1-naphthalen-2-ylethanone | C12 H10 O | 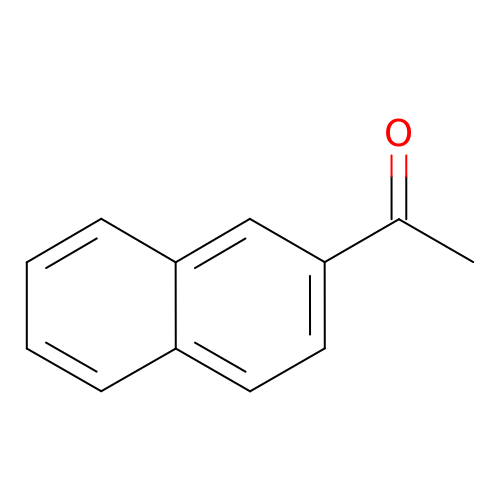XSAYZAUNJMRRIR-UHFFFAOYSA-N> EEPSDLE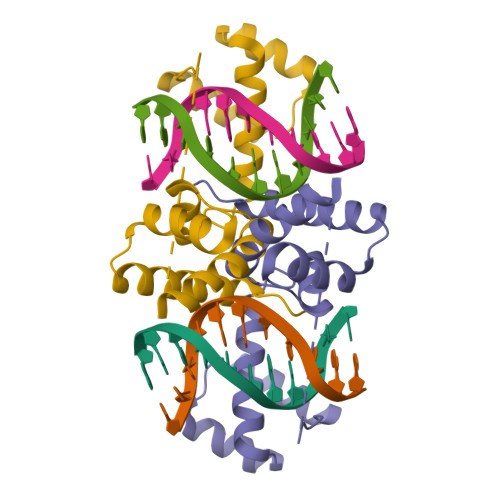ELEQFAKTFKQRRIKLGFTQGDVGLAMGKLYGNDFSQTTISRFEALNLSFKNMSKLKPLLEKWLNDAEANLSSDSSLSSPSALNSPGIEGLSRRRKKRTSIETNIRVALEKSFMENQKPTSEDITLIAEQLNMEKEVIRVWFSNRRQKEKRIN>[4x]GSHMTTRTPLMAGNWKMNLNHLEAIAHVQKLAFALADKDYDAVEVAVLAPFTDLRSVQTLVDGDKLKIKYGAQDISAHDGGAYTGEISGPMLAKLKCTYVAVGHSERRQYHAETDEIVNAKVKAAYKH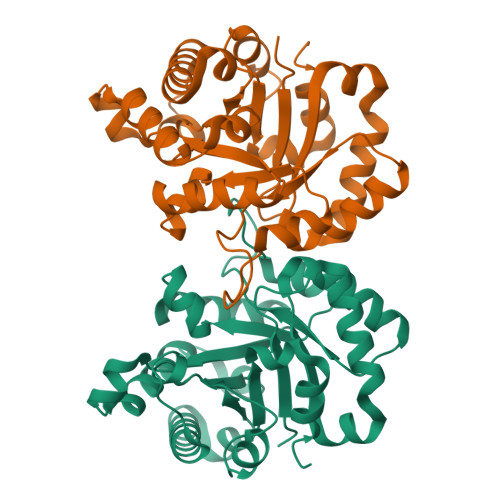GLTPILCVGEELDVREAGNHVEHTLAQVEGGLKDLAAEQAESVVIAYEPVWAIGTGKVCGADDAQEVCAAIRGKLAELYSQELADKVRIQYGGSVKSGNVAEIMAKPDIDGALVGGASLDSDEFVKIVRFRDQ4-[5-(3-chlorophenyl)-7~{H}-pyrrolo[2,3-d]pyrimidin-4-yl]morpholine 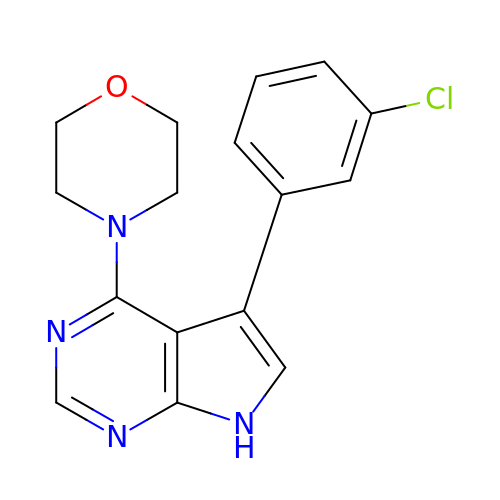| C16 H15 Cl N4 O | ONFLVQULIQDDSN-UHFFFAOYSA-N The RNA-binding protein Staufen (Stau) was originally identified in Drosophila as an mRNA transport factor required to establish the anterior–posterior axis of the embryo. In mice, the two Staufen-paralogs mStau1 and 2 share about 50% protein-sequence identity and have both been implicated in mRNA localization and RNA-dependent control of gene expression. All Stau-family proteins contain multiple so-called double-stranded RNA-binding domains (dsRBD). To probe a potential direct interaction between mStau2 and the Rgs4 mRNA, we performed in vitro binding experiments with mStau2 and the two previously predicted SRS motifs of the Rgs4 3′UTR.

EMSAs with full-length mStau2 showed binding with apparent equilibrium dissociation constants (KD) in the low micromolar concentration range for Rgs4 SRS1 as well as for SRS2. To unambiguously confirm the dsRNA fold of Rgs4 SRS2, we solved its crystal structure at 1.73 Å resolution. The RNA adopts a typical A-form double-stranded helix, characterized by a wide and shallow minor groove and a deep and narrow major groove. Whereas electron density in the stem region of both molecules is very well defined, the density map in the loop region is poor, indicating flexibility of the RNA in this region. Imino signals observed in imino 1H,1H-NOESY spectra are consistent with the base pairing observed in the crystal structure. Surprisingly, in EMSAs mStau2 dsRBD 1–2 bound the SRS2 RNA with an affinity comparable with that of dsRBD 3–4. Binding of mStau2 dsRBD 1–2 to SRS2 RNA was further confirmed by NMR titration experiments. To investigate the binding interface of mStau2 dsRBD 1–2 on SRS2 RNA, imino signals of the unbound RNA were compared with the respective resonances when bound to mStau2 at a equimolar ratio. Significant line broadening was observed in the imino signals of the four base pairs close to the stem terminus (U4, U27, U29, and G30). These were most strongly affected in the NMR spectrum of the complex, whereas other imino signals were less affected.

>[2x]ACAUGCACAUGCAAUUUGUGUAUGUGUAUGU>[2x]GSHMPIMRVASIDIGSNSVRLTIAQIKDGKLSIILERGRITSLGTKVKETGRLQ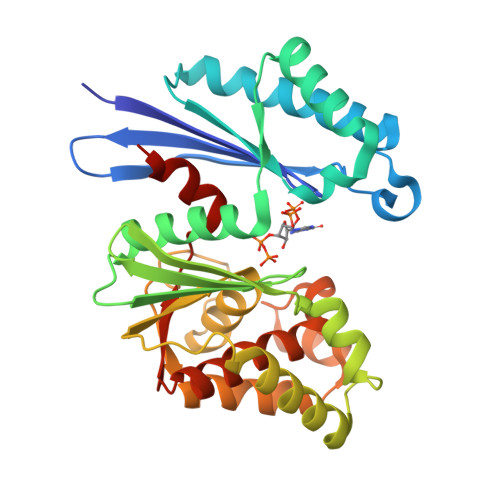EDRIEETIQVLKEYKKLIDEFKVERVKAVATEAIRRAKNAEEFLERVKREVGLVVEVITPEQEGRYAYLAVAYSLKPEGEVCVVDQGGGSTEYVFGKGYKVREVISLPIGIVNLTETFFKQDPPTEEEVKRFFEFLEKELSKVKKPVDTIVGLGGTITTLAALEYNVYPYDPQKVHGKVLTYGQIKKWFDTFKEIPSEERSKRFRQVEDRRAKVILAGIGIFLKTLEIFEKDCLIVSDWGLREGVLVSEVLKEN> EPCVEVVPNITYQCMELNFYKIPDNLPFSTKNLDLSFNPLRHLGSYSFFS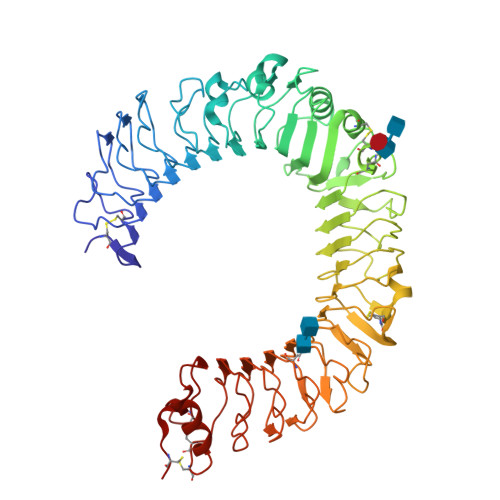FPELQVLDLSRCEIQTIEDGAYQSLSHLSTLILTGNPIQSLALGAFSGLSSLQKLVAVETNLASLENFPIGHLKTLKELNVAHNLIQSFKLPEYFSNLTNLEHLDLSSNKIQSIYCTDLRVLHQMPLLNLSLDLSLNPMNFIQPGAFKEIRLHKLTLRNNFDSLNVMKTCIQGLAGLEVHRLVLGEFRNEGNLEKFDKSALEGLCNLTIEEFRLAYLDYYLDDIIDLFNCLTNVSSFSLVSVTIERVKDFSYNFGWQHLELVNCKFGQFPTLKLKSLKRLTFTSNKGGNAFSEVDLPSLEFLDLSRNGLSFKGCCSQSDFGTTSLKYLDLSFNGVITMSSNFLGLEQLEHLDFQHSNLKQMSEFSVFLSLRNLIYLDISHTHTRVAFNGIFNGLSSLEVLKMAGNSFQENFLPDIFTELRNLTFLDLSQCQLEQLSPTAFNSLSSLQVLNMASNQLKSVPDGIFDRLTSLQKIWLHTNPWDCSCPRIDYLSRWLNKNSQKEQGSAKCSGSGKPVRSIICP> MEIAFLLNGETRRVRIEDPTQSLLEWLRAEGLTGTKEGCNEGDCGACTVMIRDAAGSRAVNACLMMLPQIAGKALRTIEGIAAPDGRLHPVQQAMIDHHGSQCGFCTPGFIVSMAAAHDRDRKDYDDLLAGNLCRCTGYAPILRAAEAAAGEPPADWLQADAAFTLAQLSSGVRGQTAPAFLPETSDALADWYLAHPEATLIAGGTDVSLWVTKALRDLPEVAFLSHCKDLAQIRETPDGYGIGAGVTIAALRAFAEGPHPALAGLLRRFASEQVRQVATIGGNIANGSPIGDGPPALIAMGASLTLRRGQERRRMPLEDFFLEYRKQDRRPGEFVESVTLPKSAPGLRCYKLSKRFDQDISAVCGCLNLT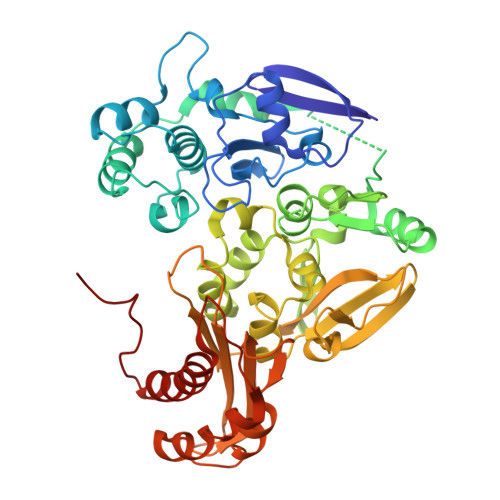LKGSKIETARIAFGGMAGVPKRAAAFEAALIGQDFREDTIAAALPLLAQDFTPLSDMRASAAYRMNAAQAMALRYVRELSGEAVAVLEVMP>MSNWVMQEENKQGNLTPLFEELLQQCPPGGQNKTAHMVSAYQLAQGNWMPTSCHVFMGTISARRTKTHPYEAYVKLRELVEEHKMKTLCPGSSLGKHNDWIIGKIKYQGNLRTKHMLNPGKVAEQLCREGHRHNVYNKTIGSVMTATGIRLEKLPVVRAQTDTTNFHQAIRDKIDKEENLQTPGLHKKLMEVFNALKRPELESSYDAVEWEELERGINRKGAAGFFERKNIGEILDSEKNKVEEIIDNLKKGRNIKYYETAIPKNEKRDVNDDWTAGDFVDEKKPRVIQYPEAKTRLAITKVMYKWVKQKPVVIPGYEGKTPLFQIFDKVKKEWDQFQNPVAVSFDTKAWDTQVTTKDLELIKDIQKYYFKKKWHKFIDTLTMHMTEVPVICADGEVYIRKGQRGSGQPDTSAGNSMLNVLTMVYAFCEATGVPYKSFDRVAKIHVCGDDGFLITERALGEKFASKGVQILAEAGKPQKITEGDKMKVAYQFDDIEFCSHTPIQVRWSDNTSSYMPGRNTTTILAKMATRLDSSGERGTIAYEKAVAFSFLLMYSWNPLIRRICLLVLSTELQVKPGKSTTYYYEGDPISAYKEVIGHNLFDLKRTSFEKLAKLNLSMSVLGAWTRHTSKRLLQDCVN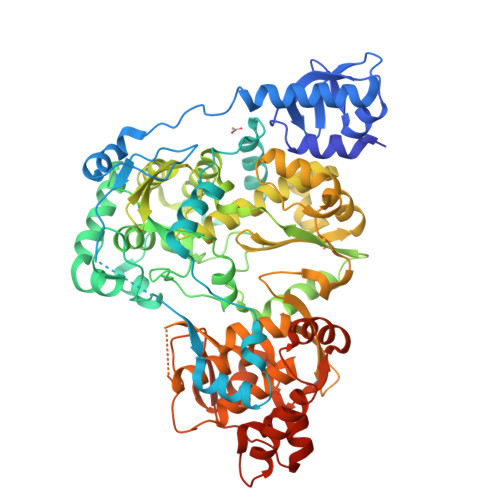MGVKEGNWLVNADRLVSSKTGNRYIPGEGHTLQGRGSSSHHHHHH[2x]>[2x]MAHHHHHHSSGLEVLFQGPAPKSGSTGKICKKTPEQLHM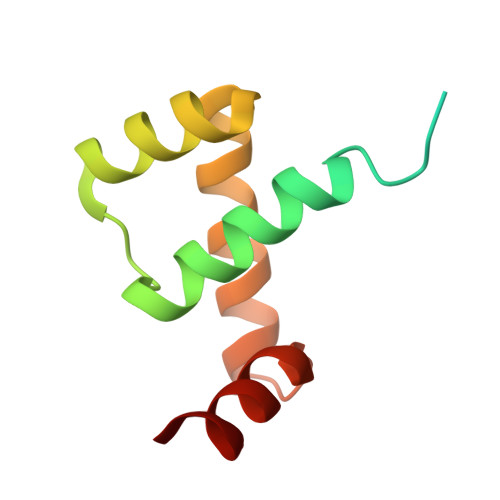LKSAFVRTQWPSPEEYDKLAKESGLARTDIVSWFGDTRYAWKNGNLKWYYYYQSANS>MSLIWKRHLTLDELNATSDNTMVAHLGIVYTRLGDDVLEAEMPVDTRTHQPFGLLHGGASAALA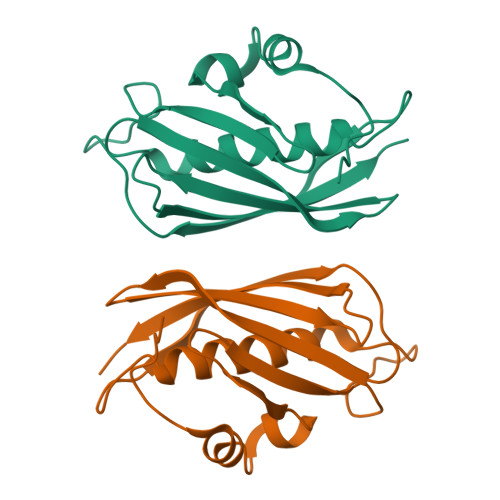ETLGSMAGFMMTRDGQCVVGTELNATHHRPVSEGKVRGVCQPLHLGRQNQSWEIVVFDEQGRRCCTCRLGTAVLGEGGSHHHHHH[2x]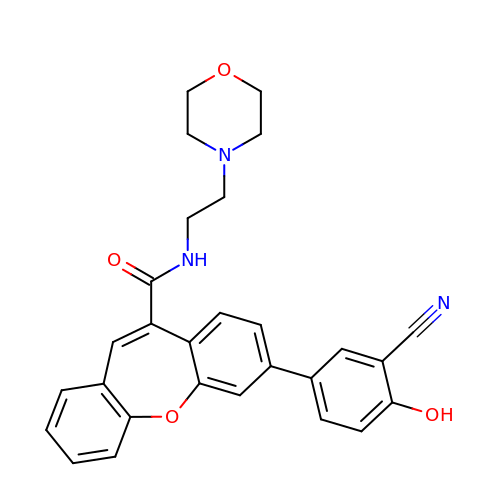7-(3-cyano-4-hydroxyphenyl)-N-[2-(morpholin-4-yl)ethyl]dibenzo[b,f]oxepine-10-carboxamide | C28 H25 N3 O4 | WKDYAACRENBHRU-UHFFFAOYSA-N>MNIVVLISGNGSNLQAIIDACKTNKIKGTVRAVFSNKADAFGLERARQAGIATHTLIASAFDSREAYDRELIHEIDMYAPDVVVLAGFMRILSPAFVSHYAGRLLNIHPSLLPKYPGLHTHRQALENGDEEHGTSVHFVTDELDGGPVILQAKVPVFAGDSEDDITA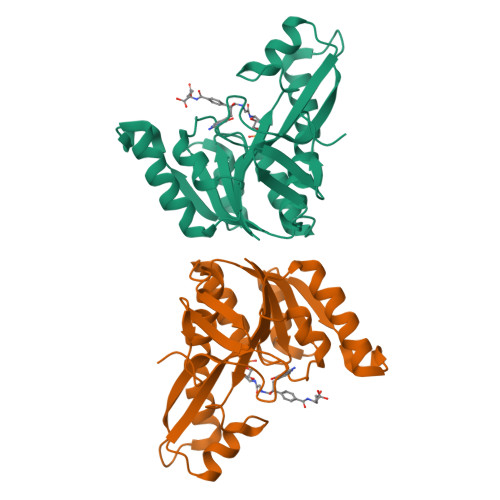RVQTQEHAIYPLVISWFADGRLKMHENAAWLDGQRLPPQGYAADE[4x]>[4x]EKYIVTWDMLQIHARKLASRLMPSEQWKGIIAVSRGGLVPGALLARELGIRHVDTVAISSYDHDNQRELKVLKRAEGDGEGFIVIDDLVDTGGTAVAIREMYPKAHFVTIFA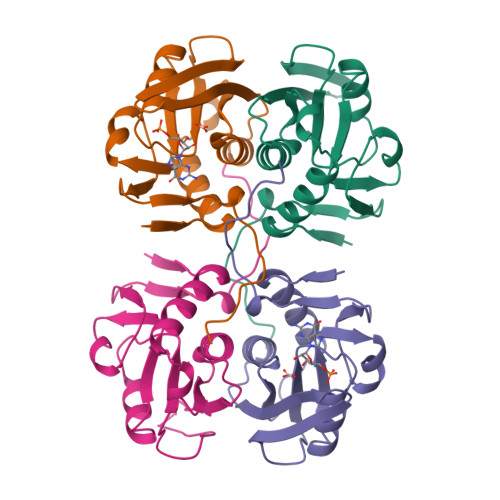KPAGRPLVDDYVVDIPQDTWIEQPWDMGVVFVPPIS> 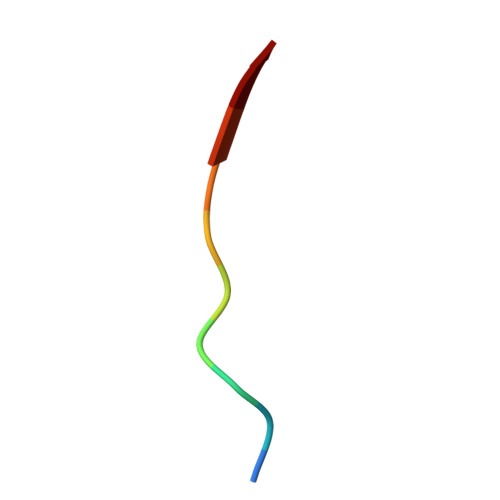GRPRTTSFAE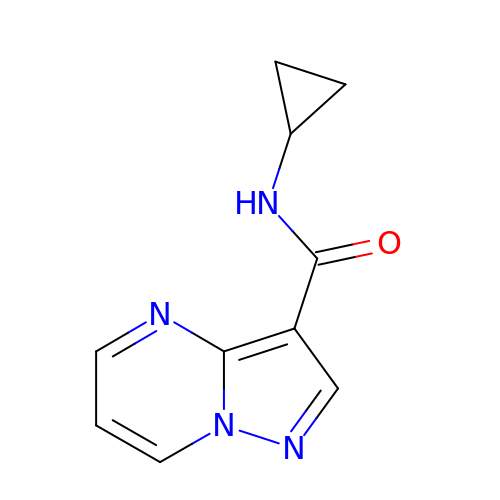N-cyclopropylpyrazolo[1,5-a]pyrimidine-3-carboxamide | C10 H10 N4 O | IDVABKGFSZEUEE-UHFFFAOYSA-N>[3x]GSSGSSGMQIGKIIKVSGPLVMAENMSEASIQDMCLVGDLGVIGEIIEMRQDVASIQVYEETSGIGPGEPVRSTGEALSVELGPGIISQMFDGIQRPLDTFMEVTQSNFLGRGVQLPALDHEKQWWFEATIEEGTEVSAGDIIGYVDETKIIQHKIMVPNGIKGTVQKIESGSFTIDDPICVIETEQGLKELTMMQKWPVRRGRPIKQKLNPDVPMITGQRVIDTFFPVTKGGAAAVPGPFGAGKTVVQHQIAKWSDVDLVVYVGCGERGNEMTDVVNEFPELIDPNTGESLMERTVLIANTSNMPVAAREASIYTGITIAEYFRDMGYDVAIMADSTSRWAEALREMSGRLEEMPGDEGYPAYLGSRLAEYYERSGRVIALGSDQREGSITAISAVSPSGGDISEPVTQNTLRVVKVFWGLDSSLAQKRHFPSINWIQSYSLYSTEVGRYMDQILQQDWSDMVTEGMRILQEEEQLNEIVRLVGIDSLSDNDRLTLEVAKSIREDYLQQNAFDDVDTFTSREKQFNMLKVILTFGKEARKALSLGAYFNEIMEGTVAVRERISRSKYIPEEELAKISSINEEIKETIQLIVSEGGMTDD;>GSSGSSGMIKEYRTIKEVVGPLMAVEKVSGVKYEELIEVRMQNGEIRRGQVLEVQEDKAMVQIFEGTSGINLKNSSVRFLGHPLQLGVSEDMIGR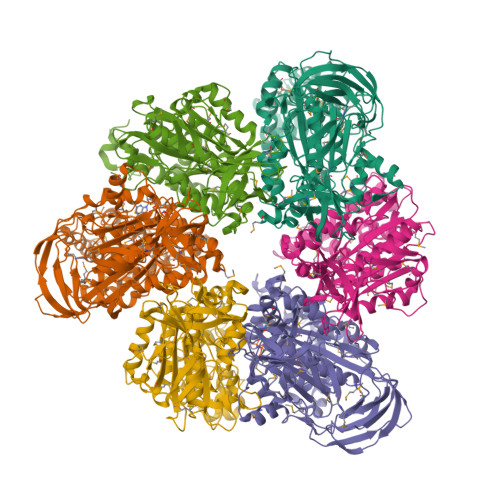VFDGLGRPKDNGPEILPEKYLDINGEVINPIARDYPDEFIQTGISAIDHLNTLVRGQKLPVFSGSGLPHKELAAQIARQATVLDSSDDFAVVFAAIGITFEEAEFFMEDFRQTGAIDRSVMFMNLANDPAIERIATPRMALTAAEYLAYEKGMHVLVIMTDMTNYAEALREISAARREVPGRRGYPGYLYTNLATLFERAGRIRGLKGSVTQIPILTMPEDDKTHPIPDLTGYITEGQIILTRELYKSGIQPPIDVLPSLSRLKDKGTGAGKTREDHAATMNQLFAAYAQGKQAKELAVVLGESALSDIDKIYAKFAERFENEYVNQGFYTNRTITETLDLGWELLAMLPRTELKRIKDDLLDKYLPEGK[3x]2'-(3-IODO-4-METHOXYPHENYL)-5-(4-METHYL-1-PIPERAZINYL)-2,5'-BI-BENZIMIDAZOLE 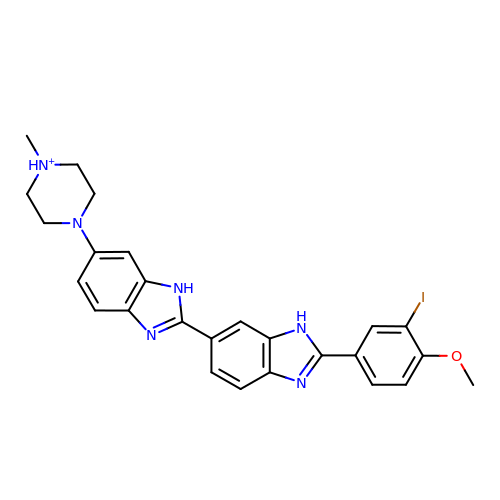| C26 H26 I N6 O | SPTCBHDLCJPQQB-UHFFFAOYSA-O> GKKSRMCGYCGAPAPYATACGLDVCVYHTHFHQHCPVIIWCGHPAGSGSCSECEPPLGKGTSPLDEVLEQVPYKPPRTVIMHVEQGLTPLDPGRYQTRRGLVSVRRGIRGNEVDLPDGDYASTALLPTCKEINMVAVASNVLRSRFIIGPPGAGKTHWLLQQVQDGDVIYTPTHQTMLDMIRALGTCRFNVPAGTTLQFPAPSRTGPWVRILAGGWCPGKNSFLDEAAYCNHLDVLRLLSKTTLTCLGDFKQLHPVGFDSHCYVFDIMPQTQL

Nsp10 belongs to the superfamily 1B (SF1B) Upf1-like family of helicases, which could unwind both DNA and RNA duplexes. In addition, this family of helicases contains an N-terminal predicted zinc-binding domain (ZBD) which is conserved in all nidovirus helicases, including 12 or 13 conserved Cys and His residues. In this paper, we present the structure of HP-PRRSV nsp10 in full length and truncation, which has a different domain arrangement compared with other helicases. The N-terminal ZBD has 13 conserved Cys/His residues, twelve of which participate in the coordination of three zinc ions.

Then we obtained crystals yielded from nsp10 incubated with a partially double-stranded DNA (dsDNA) or a single-stranded DNA (ssDNA) substrate. With the methylated nsp10 as a model, we determined the structures of full-length HP-PRRSV nsp10 and a truncated form (residues 4–273) by molecular replacement. However, no additional electron density for DNA could be identified. Comparison of these three structures showed that all the overall domain arrangement was similar, except that the truncated form lacked the C-terminal 168 residues due to the degradation during the period of crystallization.4-[2-(phenylsulfonylaminomethyl)-1,3-thiazol-4-yl]-~{N}-[3,3,3-tris(fluoranyl)propyl]benzamide | C20 H18 F3 N3 O3 S2 | 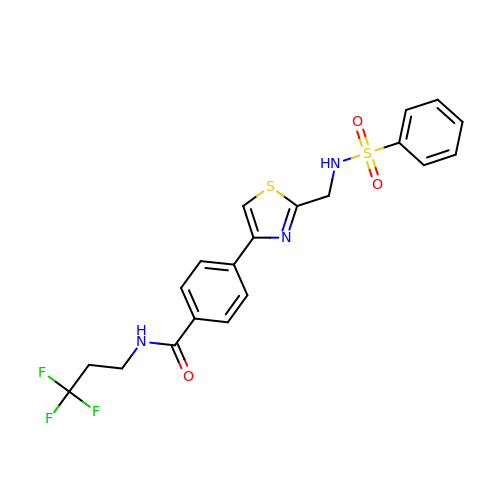WQGRXKYBROIBEJ-UHFFFAOYSA-N>DRSRVFDILSNINIGWNLGNTLDATGGGNSVNAETSWGNPKTTQEIVDTVNDRGFNAIRIPVTFANHLGPAPEYTISADWLARVKEVVDYAVNDGMYIILDTHHETNYWLKTDPNNEAALCEELAAIWKQLAEAFKDYDEKLMFEGMNEPRMAGSAKEWSGGTPAERKLINAMNKAFIDAVRATGGNNADRVLIICTYGHNSDEPTLKDLEIPSDPNIAVALHTYTPYFFTYVADGSYSVWNGSKKNDITWQYNNIKKYLIDKGIPVVITETGA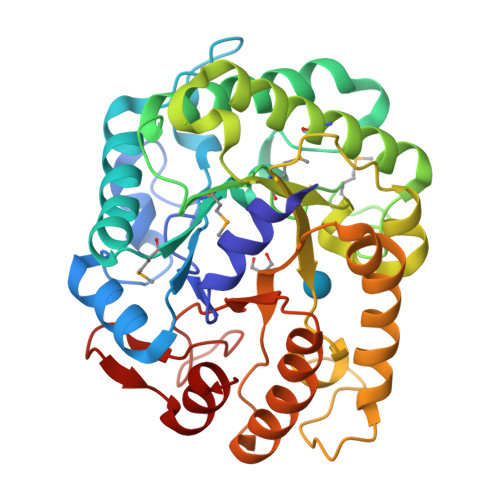QFKENTEDIVRWIGDYVGTLDQDGVKCFIWDNNIYHGNGEKFGLLNRSLLKWYNDDIVDAYVNHA[2x]>GHMEELNIDFDVFKKRIELLYSKYNEFEGSPNSLLFVLGSSNAENPYQKTTILHNWLLSYEFPATLIALVPGKVIIITSSAKAKHLQKAIDLFKDPESKITLELWQRNNKEPELNKKLFDDVIALINSAGKTVGIPEKDSYQGKFMTEWNPVWEAAVKENEFNVIDISLGLSKVWEVKDVNEQAFLSVSSKGSDKFMDLLSNEMVRAVDEELKITNAKLSDKIENKIDDVKFLKQLSPDLSALCPPNYKFNFDLLDWTYSPIIQSGKKFDLRVSARSTNDQLYGNGCILASCGIRYNNYCSNITRTFLIDPSEEMANNYDFLLTLQKEIVTNILKPGRTPKEVYESVIEYIEKTKPELVPNFTKNIGSLIGLEFRDSNFILNVKNDYRKIQR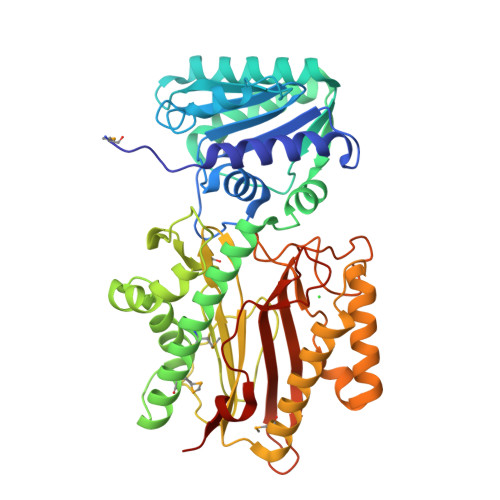GDCFNISFGFNNLKDSQSANNYALQLADTVQIPLDETEPPRFLTNYTKAKSQISFYFNNEE[2x]> GGAAUCGGAUGAAGAUAUGAGGAGAGAUUUCAUUUUAAUGAAACACCGAAGAAGUAAAUCUUUCAGGUAAAAAGGACUCAUAUUGGACGAACCUCUGGAGAGCUUAUCUAAGAGAUAACACCGAAGGAGCAAAGCUAAUUUUAGCCUAAACUCUCAGGUAAA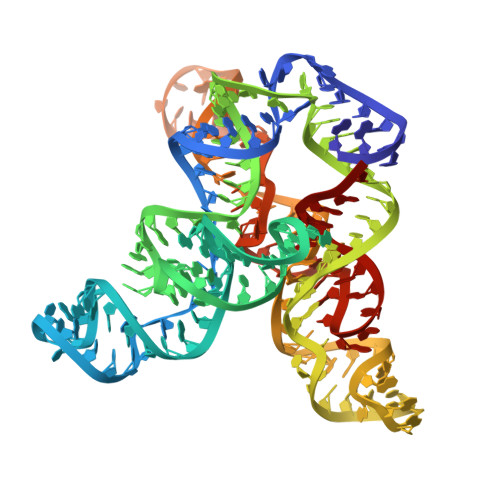AGGACGGAG> MGDSKVKVAVRVRPMNRREIDLHTKCVVDVEANKVILNPINTNLSKGDARGQPKIFAYDHCFWSMDESVREKYAGQDDVFKCLGENILQNAFDGYNACIFAYGQTGSGKSYTMMGTADQPGLIPRLCSGLFERTQKEENEEQSFKVEVSYMEIYNEKVRDLLDPKGSRQTLKVREHSVLGPYVDGLSKLAVTSYKDIESLMSEGNKSRTVAATNMNEESSRSHAVFKITLTHTLYDVKSGTSGEKVGKLSLVDLAGSERATKTGAAGDRLKEGSNINKSLTTLGLVISALADQGAGKNKNKFVPYRDSVLTWLLKDSLGGNSKTAMVATVSPAADNYDETLSTLRYADRAKHIINHAVVNEDP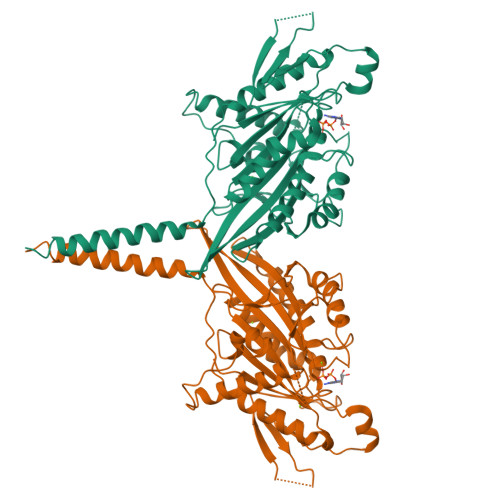NARIIRDLREEVEKLREQLTKAEAMKHHHHHH(4~{S})-6-azanyl-3-methyl-4-[3-(2-methylphenyl)-5-(trifluoromethyl)phenyl]-4-propan-2-yl-2~{H}-pyrano[2,3-c]pyrazole-5-carbonitrile 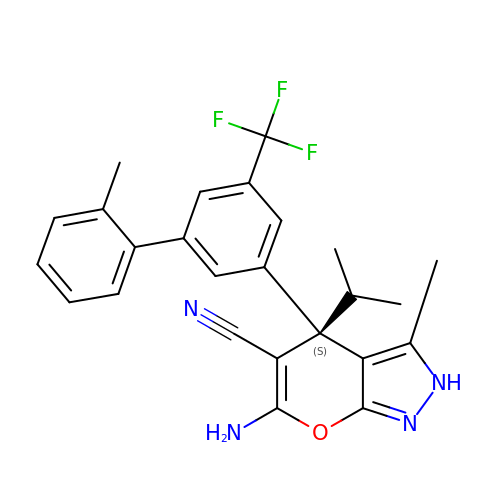| C25 H23 F3 N4 O | UBSNISIBQUMDAM-DEOSSOPVSA-N> DTIYKMNKSTRGIAVIINNKDFLRSSGMDRYPRNGTDVDR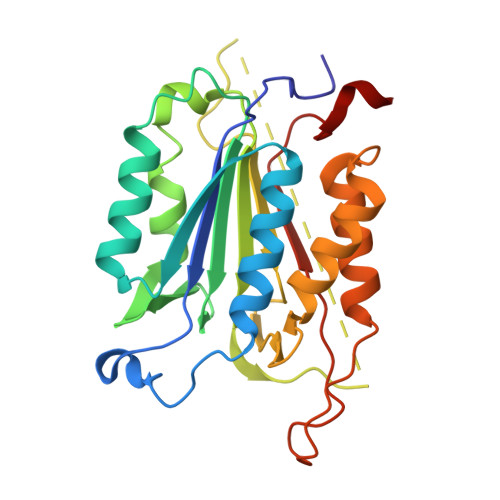DALAKLFRALKFDVRIYNNQTRAEIRRITKEMAITNHTPYDAFIFSILTHGEEGVIYGTDGTMAIKDLTAIFKDCTTLVGKPKMFFFQACQGHEYMDGVSVPAEADFVYAYSTVPGYYSWRNSVNGSWFIQSLTKVFEENAERMDILRMLTRVNAMVSTYKSRTGDYYSDSKRQVSSVVSMLRKELYFFPENV>[4x]MKHHHHHHHMHAKEGKSSEAVSQWLTAFQLQLYAPNFISAGYDLPTISRMTPEDLTAIGVTKPGHRKKIAAEISGLSIPDWLPEHKPANLAVWLSMIGLAQYY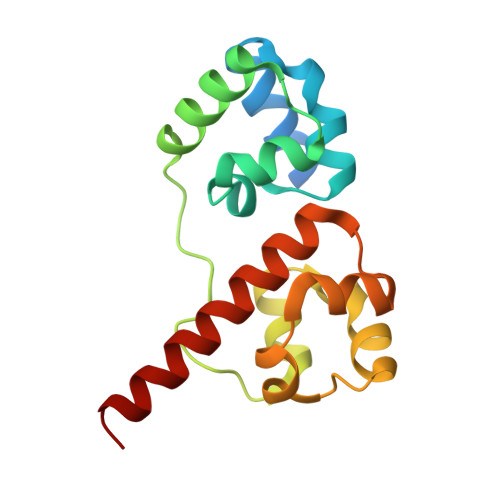KVLVDNGYENIDFITDITWEDLQEIGITKLGHQKKLMLAVRKLAELQKAEYAKY>MKRFFNRFYLDTGIIADPSQRSLASRVSAFLVQGAVAFSLLGTIGVDTSPLIAAAGVTGATIGFALKDFGTNFVASIVLSGQQSIRTGNLVCIGTGLNVVKGKVVDWDTRYLYLRSSEGHLLHVPNNMVLNSVVTWEQEKKQNPHETDLPKQDVVKAPGDNAAKQSNSLEVLFQ[7x]

Trypanosoma cruzi, the protozoan parasite causing Chagas disease, encodes a miniature MscS ortholog (TcMscS) critical for parasite development and infectivity. TcMscS contains a minimal portion of the canonical EcMscS fold yet maintains mechanosensitive channel activity, thus presenting a unique model system to assess the essential molecular determinants underlying mechanotransduction. By combining electrophysiology, single-particle cryo-EM, and all-atom molecular dynamics (MD) simulations, we show that TcMscS forms a heptameric channel with a central ion conduction path, but indeed lacks the side portals shared by other MscS-like channels. Strikingly, the presumed two TM helices are of insufficient length to fully cross an intact planar lipid membrane and thus induce drastic membrane deformation surrounding the channel.

Further examination of these TM3 kink regions allowed us to identify a point mutation, TcMscS C66L, that demonstrated higher tension sensitivity and sufficiently abolished channel inactivation in excised patches. The distinct inactivation processes occurred in the wild-type and mutant channels motivated us to also determine the cryo-EM structure of TcMscS C66L, which, surprisingly, was nearly identical to that of the wild type (root-mean-square deviations (RMSD) of ~0.4 Å for all Cα atoms, Fig. 2d). Thus, the structural basis underlying channel inactivation in TcMscS remains unclear. Nonetheless, these results demonstrate that the TM3 kink region in these MscS homologs critically regulates rates of channel inactivation and recovery. Moreover, the identical structures of the wild-type channel and a non-inactivating mutant, C66L, indicate that our cryo-EM structures unlikely represent an inactivated conformation. Inspired by these simulation results, we experimentally introduced the D47A mutation on the non-inactivating background C66L (D47A/C66L) and measured the activation pressure thresholds of C66L and D47A/C66L relative to that of the endogenous EcMscL channel. Consistently, the D47A/C66L mutant channel maintained the same unitary conductance (448.1 ± 11.5 pS, N = 5) as that of C66L, but was activated at a higher pressure threshold (PMscL/PD47A/C66L = 1.95 ± 0.51, N = 8) than C66L (PMscL/PC66L = 3.70 ± 1.24, N = 8).> PFITSR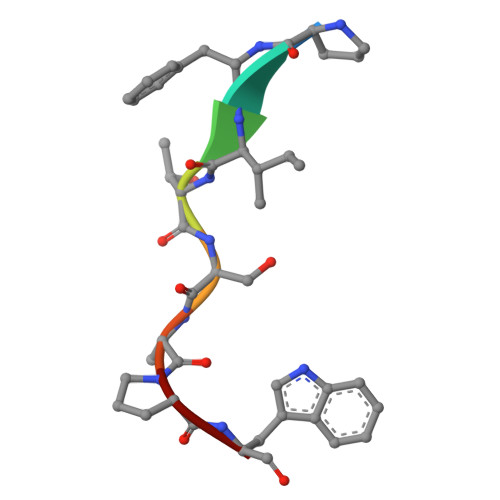PW>GAMGSSKFEEFMTRHQ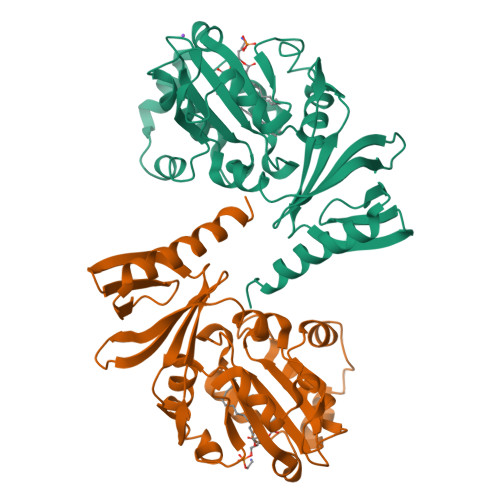VHEKEEFKALKTLSIFYQAGTSKAGNPVFYYVARRFKTGQINGDLLIYHVLLTLKPYYAKPYEIVVDLTHTGPSNRFKTDFLSKWFVVFPGFAYDNVSAVYIYNCNSWVREYTKYHERLLTGLKGSKRLVFIDCPGKLAEHIEHEQQKLPAATLALEEDLKVFHNALKLAHKDTKVSIKVGSTAVQVTSAERTKVLGQSVFLNDIYYASEIEEICLVDENQFTLTIANQGTPLTFMHQECEAIVQSIIHIRTRWELSQPD[2x]>GCTTAATTCG[2x];>CGAATTA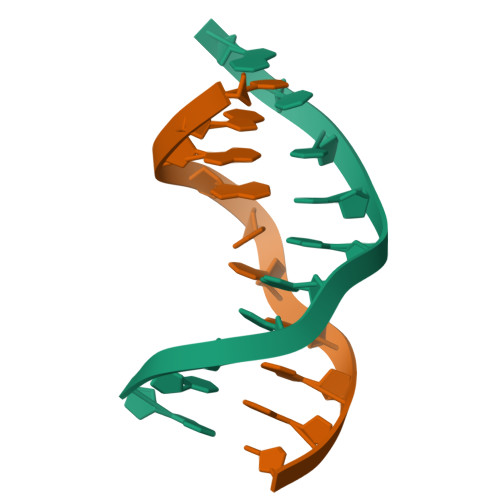AGC[2x]> AGGHGDVGMHVKEKEKNKDENKRKDEERNKTQEEHLKEIMKHIVKIEVKGEEAVKKEAAEKLLEKVPSDVLE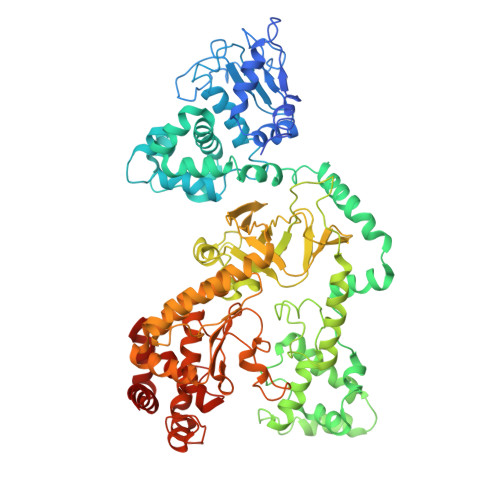MYKAIGGKIYIVDGDITKHISLEALSEDKKKIKDIYGKDALLHEHYVYAKEGYEPVLVIQSSEDYVENTEKALNVYYEIGKILSRDILSKINQPYQKFLDVLNTIKNASDSDGQDLLFTNQLKEHPTDFSVEFLEQNSNEVQEVFAKAFAYYIEPQHRDVLQLYAPEAFNYMDKFNEQEINLSLEELKDQRMLSRYEKWEKIKQHYQHWSDSLSEEGRGLLKKLQIPIEPKKDDIIHSLSQEEKELLKRIQIDSSDFLSTEEKEFLKKLQIDIRDSLSEEEKELLNRIQVDSSNPLSEKEKEFLKKLKLDIQPYDINQRLQDTGGLIDSPSINLDVRKQYKRDIQNIDALLHQSIGSTLYNKIYLYENMNINNLTATLGADLVDSTDNTKINRGIFNEFKKNFKYSISSNYMIVDINERPALDNERLKWRIQLSPDTRAGYLENGKLILQRNIGLEIKDVQIIKQSEKEYIRIDAKVVPKSKIDTKIQEAQLNINQEWNKALGLPKYTKLITFNVHNRYASNIVESAYLILNEWKNNIQSDLIKKVTNYLVDGNGRFVFTDITLPNIAEQYTHQDEIYEQVHSKGLYVPESRSILLHGPSKGVELRNDSEGFIHEFGHAVDDYAGYLLDKNQSDLVTNSKKFIDIFKEEGSNLTSYGRTNEAEFFAEAFRLMHSTDHAERLKVQKNAPKTFQFINDQIKFIINS>[3x]MATMYKPSGNKRVTFKDVGGAEEAIEELKEVVEFLKDPSKFNRIGARMPKGILLVGPPGTGATLLARAVAGEANVPFFHISGSDFVELFVGVGAARVRDLF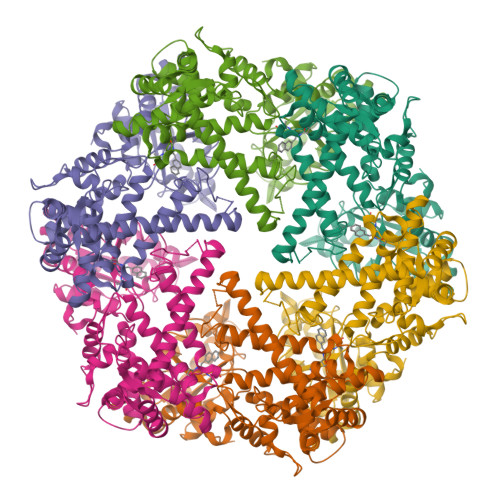AQAKAHAPCIVFIDEIDAVGRHRGAGLGGGHDEREQTLNQLLVEMDGFDSKEGIIVMAATNRPDILDPALLRPGRFDKKIVVDPPDMLGRKKILEIHTRNKPLAEDVNLEIIAKRTPGFVGADLENLVNEAALLAAREGRDKITMKDFEEAIDRVIAGPARKSLLISPAEKRIIAYHEAGHAVVSTVVPNGEPVHRISIIPRGYKALGYTLHLPEEDKYLVSRNELLDKLTALLGGRAAEEVVFGDVTSGAANDIERATEIARNMVCQLGMSEELGPLAWGKEEQEVFLGKEITRLRNYSEEVASKIDEEVKKIVTNCYERAKEIIRKYRKQLDNIVEILLEKETIEGDELRRILSEEFEKVVE> MLDNPFIGAIGYVNPDWATNVISQANQTADPTLAAQMRKVATYSTAVWLDRIAAITAGRGLRGHLDEALRQMQQAGQPVVITLVIYDLSNRDCSAAASNGELLVAQNGLARYKAEFIDPIVAILSDPRYAGLRIVTIIEPDSLPNLVTNLSIPACAEAQNAYIEGIRYAVNRLRTIPNVYIYLDIAHSGWLGWDNNFNGAVNLYTQVVQGMDQGFNSIDGFITNVANYTPFEEPYLPDPNLTIAGQPVRSASFYEWNPYFDELDYALALRNAFI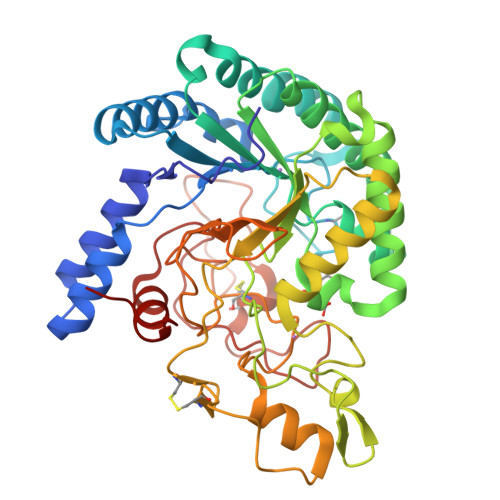GRGFPSTIGMLIDTSRNGWGGCSYGRCRPTGPSSDTSSVNAYVDGSRVDRRYHRGNWCNQAGGIGERPQAAPRSGIDAYVWVKPPGESDGVSQPGIVDPDDPNKKFDPMCDPNGQSRYNSAYPTGALPNAPHAGRWFPQQSEILVRNAYPPIQP>[2x]MFQTVTILLDWFGLCIFTVTGALVASRKEMDIA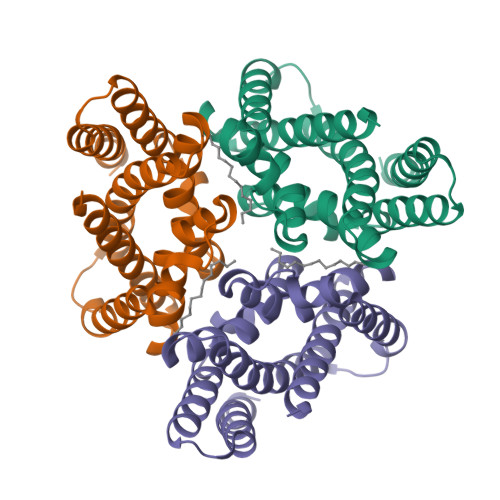GFVLLGAVTGVGGGTIRDLVLGRTPVFWVEEPAYVLACLGVAVFTFFFAHIPQSRYRFLLWLDAVGLSLFAVTGAERALQTGAGPVIAIAMGVATATFGGILRDLLGGESPVILRREIYITAALLGAAAFVALDAFGAPRELALGAGFAAAFLSRAAGLVWGLSLPRYRARLESSGENLYFQ> GSEDLPHHDEKTWNVGSSNRNKAENLLRGKRDGTFLVRESSKQGCYACSVVVDGEVKHC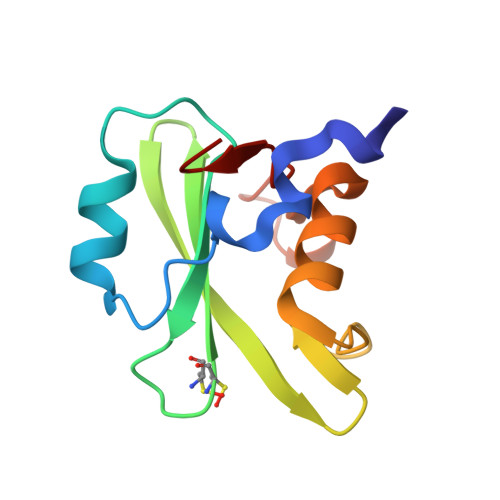VINKTATGYGFAEPYNLYSSLKELVLHYQHTSLVQHNDSLNVTLAYPVYA>AEGPAKKVLTLEGDLVLGGLFPVHQKGGPAEDCGPVNEHRGIQRLEAMLFALDRINRDPHLLPGVRLGAHILDSCSKDTHALEQALDFVRASLSRGADGSRHICPDGSY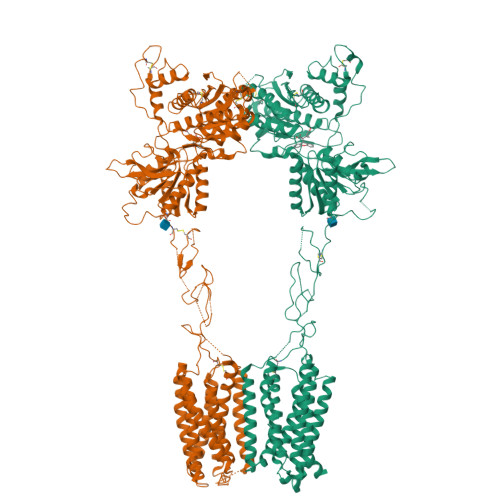ATHGDAPTAITGVIGGSYSDVSIQVANLLRLFQIPQISYASTSAKLSDKSRYDYFARTVPPDFFQAKAMAEILRFFNWTYVSTVASEGDYGETGIEAFELEARARNICVATSEKVGRAMSRAAFEGVVRALLQKPSARVAVLFTRSEDARELLAASQRLNASFTWVASDGWGALESVVAGSEGAAEGAITIELASYPISDFASYFQSLDPWNNSRNPWFREFWEQRFRCSFRQRDCAAHSLRAVPFEQESKIMFVVNAVYAMAHALHNMHRALCPNTTRLCDAMRPVNGRRLYKDFVLNVKFDAPFRPADTHNEVRFDRFGDGIGRYNIFTYLRAGSGRYRYQKVGYWAEGLTLDTSLIPWASPSAGPLPASRCSEPCLQNEVKSVQPGEVCCWLCIPCQPYEYRLDEFTCADCGLGYWPNASLTGCFELPQEYIRWGDAWAVGPVTIACLGALATLFVLGVFVRHNATPVVKASGRELCYILLGGVFLCYCMTFIFIAKPSTAVCTLRRLGLGTAFSVCYSALLTKTNRIARIFGGAREGAQRPRFISPASQVAICLALISGQLLIVVAWLVVEAPGTGKETAPERREVVTLRCNHRDASMLGSLAYNVLLIALCTLYAFKTRKCPENFNEAKFIGFTMYTTCIIWLAFLPIFYVTSSDYRVQTTTMCVSVSLSGSVVLGCLFAPKLHIILFQPQKNVVSHRAPTSRFGSAAARASSSLGQGSGSQFVPTVCNGREVVDSTTSSL[2x]>GGSEAVSDIYKPFWEWAAKTIKERLGDDLVSYPIPDGYLRKEAMVGKGKRESLAWTQSYGYQTKKMRQIRAAHVNGGASLQVLNLVFFPHMNYDLPFLGLDLVTLPGGHLIAIDMQPLFQTEEYKKKYAEPCMDMYQKHVKNLPWGGDFPEEAKQYFSPVFLWTRPQEDKQVETYVFEAFKDYINKYLDFVEAAKPVTDPDHLARIRERQLSYLQYRAEKDP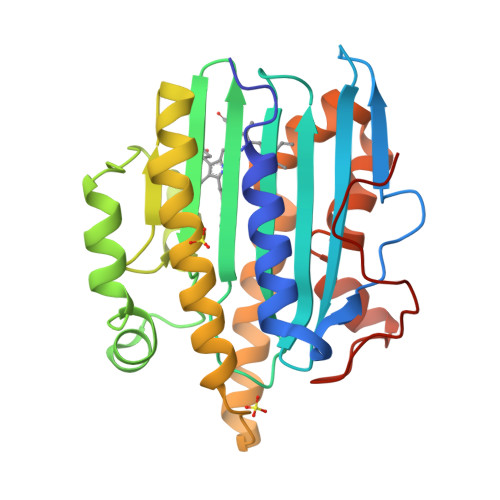ARGMFTRMYGPEWTERYIHGFLFDLEEKMESGEYKTGELLPCSDPLNFQPTPL[2x]> GSSKKVGTLNRFTQALVIAYVIGYVFVYNKGYQDTDTVLSSVTTKVKGIALTKTSELGERIWDVADYIIPPQEDGSFFVLTNMIITTNQTQSKCAENPTPASTCTSHRDCKRGFNDARGDGVRTGRCVSYSASVKTCEVLSWCPLEKIVDPPNPPLLADAERFTVLIKNNIRYPKFNFNKRNILPN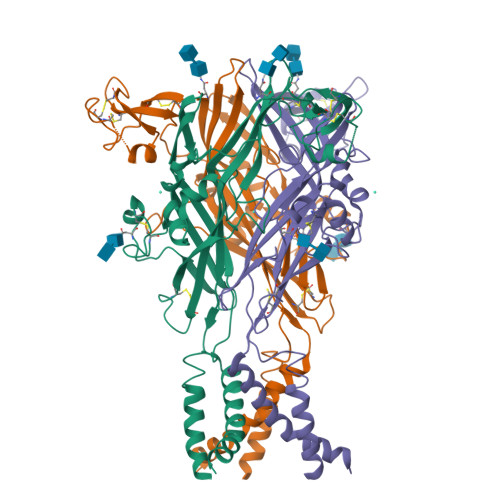INSSYLTHCVFSRKTDPDCPIFRLGDIVGEAEEDFQIMAVRGGVMGVQIRWDCDLDMPQSWCVPRYTFRRLDNKDPDNNVAPGYNFRFAKYYKNSDGTETRTLIKGYGIRFDVMVFGQAGKFNIIPTLLNIGAGLALLGLVNVICDWIVLTFMKRKQHYKEQKYTYVDDF> MATTTVGLTDLKVRLVRDDFADAVAWVARSLPSRPTVPVLAGVLLTGSDDGLTISSFDYEVSAEVQIPAEIAAPGTVLVSGRLLSEITRALPNKPVDLSVEGTRVSLTCGSARFSLPTMAVEDYPALPELPAETGSVPADLFAEAIGQVAVAAGRDDTLPMLTGIRVEISGDRMVLAATDRFRLAVRELTWTTKTPDVEAAVLVPAKTLAEAAKTGLDGSEVQLALGAGPSVGQDGLLGIRSEGKRSTTRLLDAEFPKFRQLLPTEHTAMATIGVGELTEAIKRVALVADRGAQVRMEFADDVLHLSAGADDVGRAEEDLPVSFSGEPLTIAFN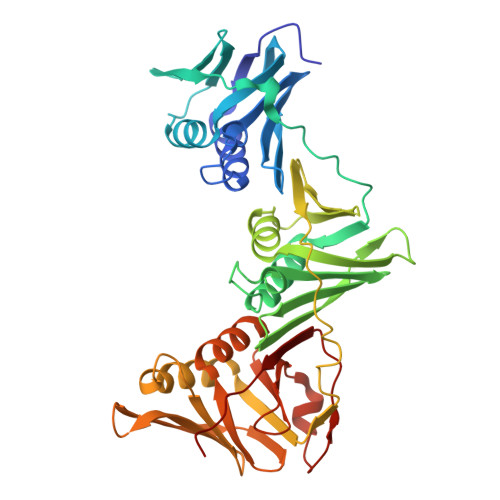PGYLTDGLGALHSERVTFGFTTPSKPAVLRPATEADAALNGNGPFPAAETDYVYLLMPVRLPG> TMVDQAVMDKLDAGFKKLQAANECHSLLKKHLTKDIYDQLKCKKTDMGATLLDVVQSGMENLDSGVGIYAPDAQAYKTFSALFDPIIDDYHKGFKPTDKHPKTDFGDLNYFVNVDPKNEYVISTRVRCGRSLQGYPFNPMLTEAQYKEMEDKVKAQLATFDGELKGTYYPLLGMDKATQQKLIDDHFLFKEGDRFLQAANACRYWPVGRGIFHNDKKTFLMWVNEEDHLRIISMQKGGDLKEVYGRLVK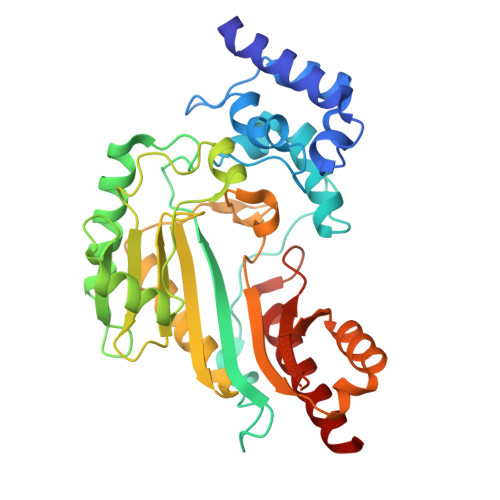AVQHIEKKIPFSRDDRLGFLTFCPTNLGTTIRASVHIKLPKLAADRKKLEEVAARYNLQVRGTAGEHTESVGGVYDISNKRRMGLTEFQAVKEMQDGILELIKIEKSL> NEDMPVERILEAELAVEPKTETYVEANMGLNPSSPNDPVTNICQAADKQLFTLVEWAKRIPHFSELPLDDQVILLRAGWNELLIASFSHRSIAVKDGILLATGLHVHRNSAHSAGVGAIFDRVLTELVSKMRDMQMDKTELGCLRAIVLFNPDSKGLSNPAEVEALREKVYASLEAYCKHKYPEQPGRFAKLLLRLPALRS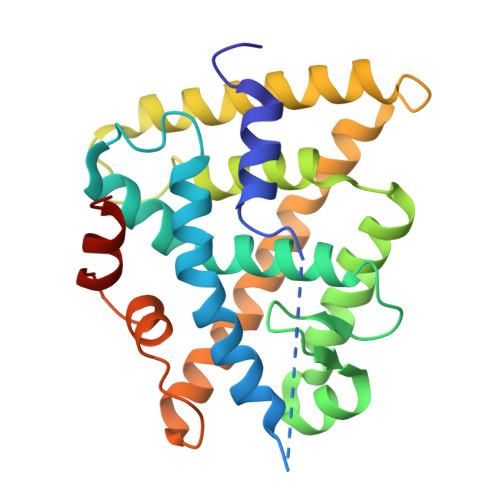IGLKCLEHLFFFKLIGDTPIDTFLMEMLEAPHQMTGGSGGSSHSSLTERHKILHRLLQEGSPS S-(2-oxo-2-phenylethyl) (2R)-2-benzyl-4,4,4-trifluorobutanethioate 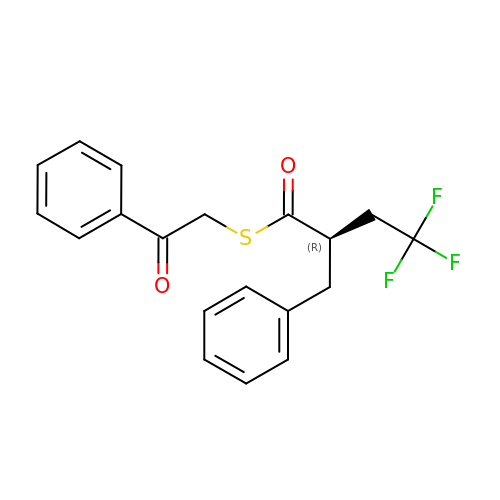| C19 H17 F3 O2 S | CADIQQIULRUWPM-MRXNPFEDSA-N>[6x]MGSSHHHHHHSSGENLYFQGSQQFPQFHVKSGLQIKKNAIIDDYKVTSQVLGLGINGKVLQIFNKRTQEKFALKMLQDCPKARREVELHWRASQCPHIVRIVDVYENLYAGRKCLLIVMECLDGGELFSRIQDRGDQAFTEREASEIMKSIGEAIQYLHSINIAHRDVKPENLLYTSKRPNAILKLTD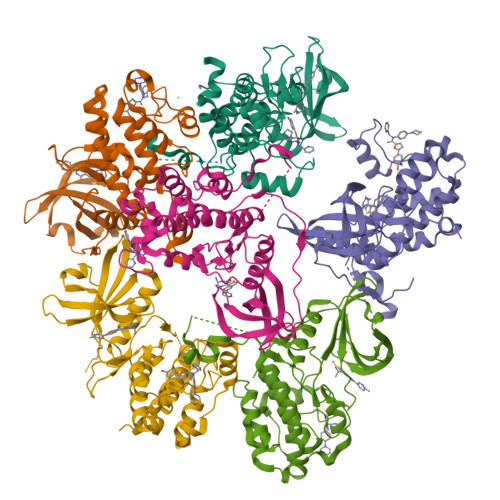FGFAKETTSHNSLTEPCYTPYYVAPEVLGPEKYDKSCDMWSLGVIMYILLCGYPPFYSNHGLAISPGMKTRIRMGQYEFPNPEWSEVSEEVKMLIRNLLKTEPTQRMTITEFMNHPWIMQSTKVPQEPLHT> MNKAKIFMNGQSQA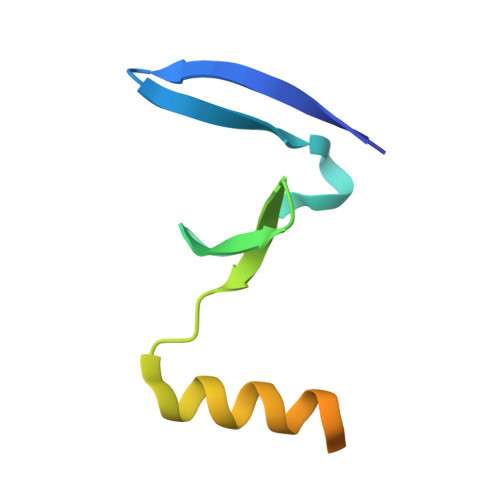VRLPKEFRFSVKEVSVIPLGKGIVLQPLPNSWKDVFQEMAEISSDDIFPEGRKDLPPQKRKYFE>KETTSFVFTRFSPDPQNLLLQGDTVVTSSGHLQLTQVKDGEPVYSSLGRALYYAPIHIWDSNTDTVANFVTSFSFVIDAPNKAKAADGLAFFLAPVDTEPQKPGGLLGLFHDDRHNKSNHIVAVEFD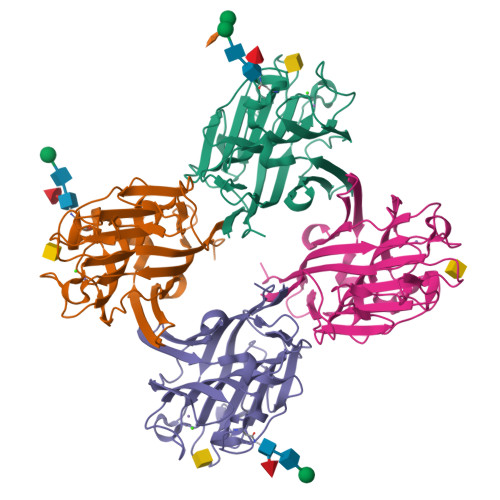TFKNSWDPEGTHIGINVNSIVSRKTISWDLENDEVANVVISYQASTKTLTASLVYPSSSTSYILNDVVDLKQILPEYVRVGFTAASGLSKDHVETHDVLAWTFDSDLPDPSSDDCN[4x]>[3x]TEIVCDKTVEVVKNAIETADGALDLYNKYLDQVIPWQTFDETIKELSRFKQEYSQAASVLVGDIKTLLMDSQDKYFEATQTVYEWAGVATQLLAAYILLFDEYNEKKASAQKDILIKVLDDGITKLNEAQKSLLVSSQSFNNASGKLLALDS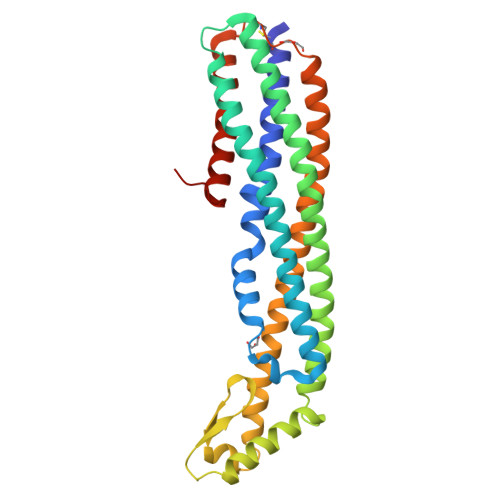QLTNDFSEKSSYFQSQVDKIRKEAYAGAAAGVVAGPFGLIISYSIAAGVVEGKLIPELKNKLKSVQNFFTTLSNTVKQANKDIDAAKLKLTTEIAAIGEIKTETETTRFYCDYDDLMLSLLKEAAKKMINTANEYQKRHGKKTLFEVPEV Successive assemblies of Endosomal Sorting Complexes Required for Transport (ESCRT-I, -II and III) largely mediate sorting of plasma membrane receptors at endosomal membranes, the formation of multivesicular bodies and their release into the endosomal lumen. ESCRT-I subsequently recruits ESCRT-II, composed of Vps22, Vps25, and Vps36, which in turn activates ESCRT-III subcomplexes. Two recent crystal structures of a core of the ESCRT-II complex reveal a trilobal complex, containing two copies of Vps25, one copy of Vps22 and the C-terminal region of Vps36. The human and rat homologues of ESCRT-II were originally identified as the EAP complex (ELL Associating Protein; Vps22/EAP30; Vps25/EAP20; Vps36/EAP45), associated with the RNA polymerase II elongation factor ELL in the nucleus.

Here, we report the crystal structure of full-length yeast Vps25, composed of two homologous winged-helix domains. Vps25 consists of two homologous winged helix domains as detected by the program GRATH that are arranged in tandem. The N-terminal domain 1 (residues 1 to 126) contains two additional N-terminal 3/10 helices, implicated in the interaction with either Vps22 or Vps36, followed by the canonical helix 1 and strand 1. It lacks canonical helix 2, which instead folds into a large disordered loop followed by strands 3 and 4 that connects to helix 2 (at the corresponding position of canonical helix 3). Domains 1 and 2 are tightly packed against each other and their C alpha atoms can be superimposed with an r.m.s. deviation of 3.4 Å, confirming their structural relatedness. In the unliganded Vps25 structure, this helical segment constitutes the 1192 Å2 dimerization interface of two identical Vps25 dimers present in the asymmetric crystal unit. The dimer contact is mediated by hydrophobic residues Pro5, Pro6, Val7, Phe10, Pro11, and Pro12, which is similar to the contact region described for Vps25 interactions with Vps22 and Vps36. In the Vps25 structure Arg83 does not participate in dimerization but hydrogen bonds to Thr15 instead of forming salt bridges with either Vps36 Asp548 or Vps22 Asp214 as observed in the ESCRT-II complex. Therefore Vps25 seems to dock as a rigid body onto either Vps22 or Vps36 upon ESCRT-II complex formation. Surface electrostatic potential maps of Vps25 reveal a negatively charged surface within domain 2 that is characterized by a patch of conserved residues such as Glu153, Glu170 and Tyr152.

>[4x]MSALPPVYSFPPLYTRQPNSLTRRQQISTWIDIISQYCKTKKIWYMSVDGTVINDNELDSGSTDNDDSKKISKNLFNNEDIQRSVSQVFIDEIWSQMTKEGKCLPIDQSGRRSSNTTTTRYFILWKSLDSWASLILQWFEDSGKLNQVITLYELSEGDETVNWEFHRMPESLLYYCLKPLCDRNRATMLKDENDKVIAIKVV>DNPGTAPLDTF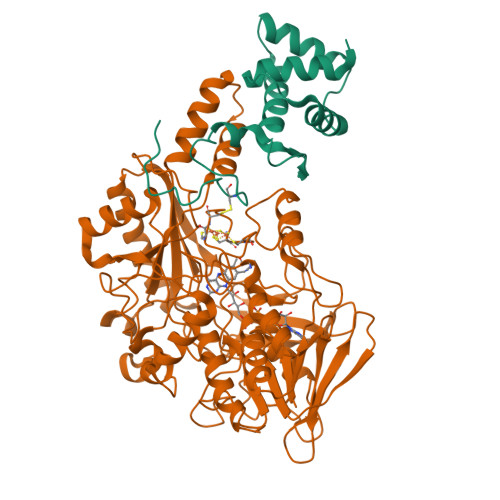MTLSESLTGKKGLSRVIGERLLQALQKGSFKTADSLPQLAGALASGSLTPEQESLALTILEAWYLGIVDNVVITYEEALMFGVVSDTLVIRSYCPNKPGFWADKPIERQA[2x];>[2x]MADTDTQKADVVVVGSGVAGAIVAHQLAMAGKAVILLEAGPRMPRWEIVERFRNQPDKMDFMAPYPSSPWAPHPEYGPPNDYLILKGEHKFNSQYIRAVGGTTWHWAASAWRFIPNDFKMKSVYGVGRDWPIQYDDLEPYYQRAEEELGVWGPGPEEDLYSPRKQPYPMPPLPLSFNEQTIKTALNNYDPKFHVVTEPVARNSRPYDGRPTCCGNNNCMPICPIGAMYNGIVHVEKAERAGAKLIENAVVYKLETGPDKRIVAALYKDKTGAEHRVEGKYFVLAANGIETPKILLMSANRDFPNGVANSSDMVGRNLMDHPGTGVSFYASEKLWPGRGPQEMTSLIGFRDGPFRATEAAKKIHLSNLSRIDQETQKIFKAGKLMKPDELDAQIRDRSARYVQFDCFHEILPQPENRIVPSKTATDAIGIPRPEITYAIDDYVKRGAAHTREVYATAAKVLGGTDVVFNDEFAPNNHITGSTIMGADARDSVVDKDCRTFDHPNLFISSSATMPTVGTVNVTLTIAALALRMSDTLKKEVHHHHHH>[2x]GFEDFNTNP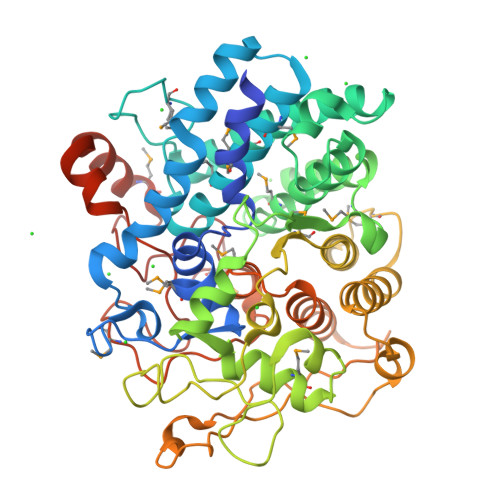YQPSKVPASNLLSTMFNVYACPQQNACQEINCMWASFSGQVTATANWSFGKNIFAYYNASEGHNDSSWGRLYGYIYPSFFLVENSTEKKGVIYAMAQLTRVYGMQLLASLQGPIPYTQMKAGETEAPYDNEQTVWHAMFDDLDNAITILKSAATFGVNQDLAVVDQFYKGDCSKWLKFANTLKLRMAIRISGVEPEYAQTKAQEAVLGGVMESVGDSSYDTTNGGINENGYAIVSGWPEVRANACLVSYMNGYNDPRRPAYFTPQTQTAAGGYVGVRSGSAEIPEPTVYANYSKLFIATDKTLPQPVMYAAEAAFLRAEGALKGWNMGGDAKTFYEKGVRLSFEEFGVSGADDYLADATSIPGNYVDNLIAGHTGNNYTNQSSITIKWEDGADDAKKLERVLTQKWIACYPDPMNGWADFRRTGYPRIFPATESMNADCNTGRGQRRLRFTRSEYNNNKANVEAAVSMLSNGKDSNGTDLWWAMKENGTY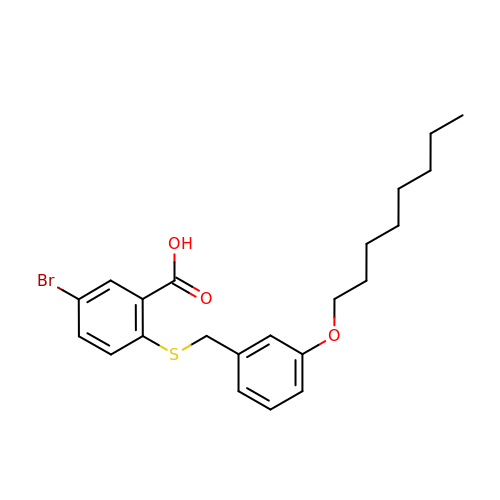5-bromo-2-{[3-(octyloxy)benzyl]sulfanyl}benzoic acid | C22 H27 Br O3 S | DMCLNIZKWQGPTM-UHFFFAOYSA-N>SFSNFPISEETIKLLKGRGVTFLFPIQAKTFHHVYSGKDLIAQARTGTGKTFSFAIPLIEKLHGELQDRKRGRAPQVLVLAPTRELANQVSKDFSDITKKLSVACFYGGTPYGGQFERMRNGIDILVGTPGRIKDHIQNGKLDLTKLKHVVLDEVDQMLDMGFADQVEEILSVAYKKDSEDNPQTLLFSATCPHWVFNVAKKYMKSTYEQVDLIGKKTQKTAITVEHLAIKCHWTQRAAVIGDVIRVYSGHQGRTIIFCETKKEAQELSQNSAIKQDAQ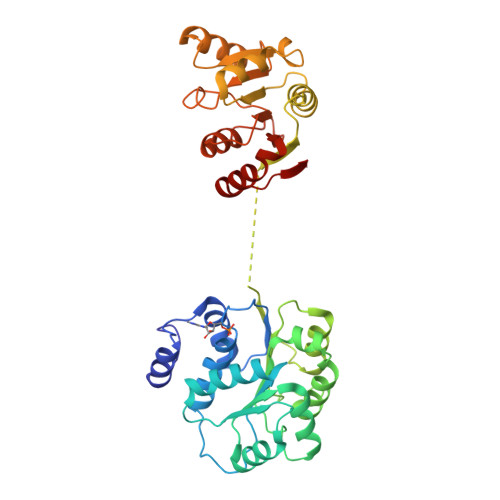SLHGDIPQKQREITLKGFRNGSFGVLVATNVAARGLDIPEVDLVIQSSPPKDVESYIHRSGRTGRAGRTGVCICFYQHKEEYQLVQVEQKAGIKFKRI[5x]> MNRFFKVSSKYQYYKYLEQYDAAFLRKYQSETHWYLGRRGAWKNLVIKYAGDHISLEEEHNVKYKTHLSFVYLSYRLAWVLFAYVLIYNHFLLGDIGKTFNVG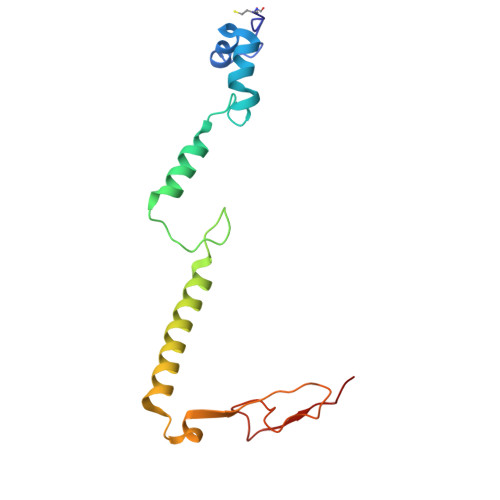EWDHRLKPSAERDYPTRYESLYILDRTQKW3-[(4-cyanobenzyl)amino]-6-(trifluoromethyl)quinoxaline-2-carboxylic 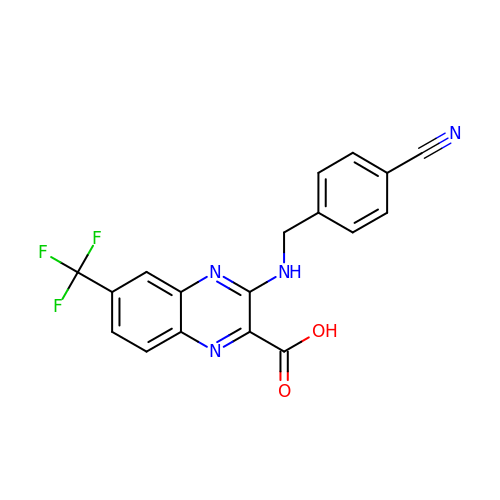acid | C18 H11 F3 N4 O2 | RFEBDZANCVHDLP-UHFFFAOYSA-N>[8x]MKKTKIVCTIGPKTESEEMLAKMLDAGMNVMRLNFSHGDYAEHGQRIQNLRNVMSKTGKTAAILLDTKGPEIRTMKLEGGNDVSLKAGQTFTFTTDKSVIGNSEMVAVTYEGFTTDLSVGNTVLVDDGLIGMEVTAIEGNKVICKVLNNGDLGENKGVNLPGVSIALPALAEKDKQDLIFGCEQGVDFVAASFIRKRSDV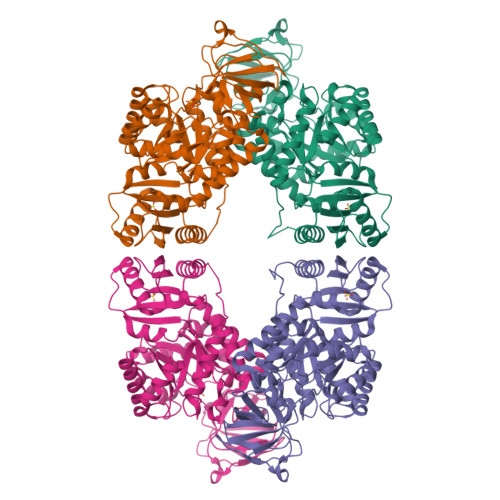IEIREHLKAHGGENIHIISKIENQEGLNNFDEILEASDGIMVARGDLGVEIPVEEVIFAQKMMIEKCIRARKVVITATQMLDSMIKNPRPTRAEAGDVANAILDGTDAVMLSGESAKGKYPLEAVSIMATICERTDRVMNSRLEFNNDNRKLRITEAVCRGAVETAEKLDAPLIVVATQGGKSARAVRKYFPDATILALTTNEKTAHQLVLSKGVVPQLVKEITSTDDFYRLGKELALQSGLAHKGDVVVMVSGALVPSGTTNTASVHVL>[2x]MAHHHHHHVDDDDKMAQGLKDAYKD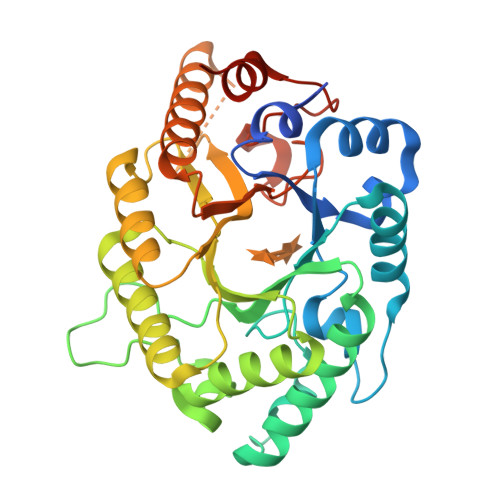YFKIGVAVNNRNVADPDQIKVVLREFNSITAENAMKPQPTEPKKGEFNWEDADKIADFCRANGIKMRGHTLMWHSQIGSWMYQDEKGNLLSKEEFYANMKHHIQAIVNRYKDVVYCWDVVNEAVADSPVYPGRPELRNSPMYQIAGEEFIYKAFEYAHEADPDALLFYNDYNDAEPAKSQRIYNLVKRMKDAGVPIDGIGMQAHYNVYGPTMKEVDDAIKLYSTVVDHIHLTELDIRINEDMGGGLRFNQGQATVSDWERTLQQDQYVQLFKVLRKHKDVIDCVTFWNVSDKDSWLGVRNYPLLFDENYKPKQAYNAVKNFDPKMDNAVI>[2x]MMASAATELDVDGVKVRFTNPDKVYFPKLGKNGTKGKLVEYYLSVASGPMLALLRDRPVHLQRFPDGIEGEEIYQKRVPQKHPDYLETCVVTFPSGRTADALKITHPSSIIWAAQMGTVTLHPWQVRCPDTEHPDELRVDLDPQPGTGFKEARTVACDVLKPLLDELGLVGYPKTSGGRGVHVFLRIKPQWDFIEVRRAGIALAREVERRAPDAVTTSWWKEERGERLFIDYNQNARDRTFASAYSVRKTPIATVSMPLSWDELRNADPDDYTMNTVPDLLAGRDDPWADIDSVQQSLGPLLDLVAADEERGLGDLPYPPNYPKMPGEPPRVQPSKKVAEHWDEQGNRKQ

Recently, it was reported that a closely related enzyme called Prim–PolC, operonically associated with ligase C (LigC), is specifically involved in LigC-dependent repair of short DNA-gapped intermediates produced during excision-repair processing of lesions in mycobacteria, further expanding the repertoire of pathways in which these diverse replicases operate. A notable feature of Prim–PolC is its favourable activity on short DNA gaps of 1–3 nucleotides, which it preferentially fills in with ribonucleotides. Although the crystal structure of the apo Prim–PolC showed that it is remarkably similar to Prim–PolD, it contains a unique C-terminal extension called Loop 3, proposed to be potentially involved in gap recognition. To understand the molecular basis for its gap-binding and synthesis activities, we elucidated the crystal structures of pre- and post-catalytic intermediates of Prim–PolC bound to DNA substrates containing a two-nucleotide gap.

To elucidate the structural transitions that occur during Prim–PolC’s catalytic cycle, we next crystallised a post-catalytic 1-nt gap ternary complex by mixing Prim–PolC, 2-nt gap DNA, Mn2+ and a 3′-deoxy chain-terminating ribonucleotide, 3′-dUTP (3′-dUTP is UTP lacking a 3′-hydroxyl group). The structure revealed that the expected turnover reaction had occurred, as an incorporated ribonucleotide was now visible on the 3′ end of the primer strand, leaving a 1-nt gap. Further turnover was not possible due to the lack of a 3′-OH moiety on the newly extended primer strand. The crystals contained two complexes in the asymmetric unit and, fortuitously, each of these complexes represents a different post-catalytic intermediate state. In one complex, the active site is occupied with inorganic pyrophosphate (PPi), the remnants of the previous nucleotidyl transfer reaction. R179 effectively creates a gate that is observed in the ‘closed’ position, thus preventing PPi from leaving the active site. In the other complex in the asymmetric unit, we observed the next step in the enzymatic pathway, the binding of the next incoming rNTP into the active site, following PPi release. The R179 ‘gate’ is in the open position, presumably to allow PPi to leave the active site to facilitate the binding of the next incoming nucleotide. The DNA has undergone a frameshift translation in the upstream direction, resulting in a loss of engagement of the upstream duplex with Loops 2 and 3. This disengagement is promoted by the increased splaying angle of the bases (111.6°) at the hydrophobic wedge I73/Y74, a difference of ∼14.3° compared with the pre-turnover complex.> SNAMSPEALQVRDAEDADWPAILPFFREIVSAGETYAYDPELTDEQARSLWMTPSGAPQSRTTVAVDADGTVLGSANMYPN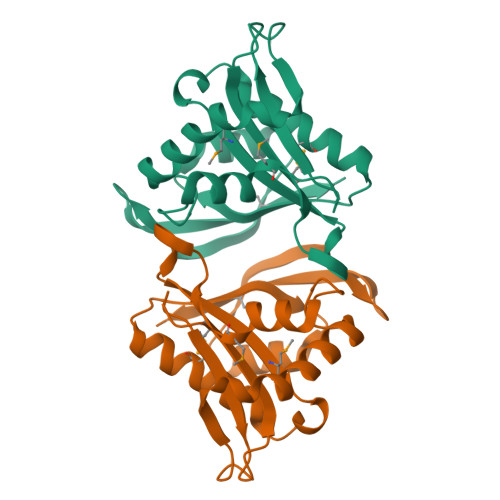RPGPGAHVASASFMVAAAARGRGVGRALCQDMIDWAGREGFRAIQFNAVVETNTVAVKLWQSLGFRVIGTVPEAFHHPTHGYVGLHVMHRPL>AMALTGCSEKININEDKISHKIDIPDSAWTIGIGEKFKNAGHPNVKYPMIDDSYVQGAPLGGFGAGTIGRTYNGGFSRWHLEIGKNKYTTVYANQFSVFQKVEGNKDGVAQVLYAGEPENGYLSSWKWDYPKESGMYYALYPNSWYTYTNKDLPVQLAVKQFSPIIPYNYKETSYPVAVFKWTAYNPTNKNVDVSIMFTWQNMIGFFGKQVNVNSGNFNKIIKDKSKDSEIVAAVMGNISNDNEEWNGEYSIGVKKVPGVDISYKAKFVTTGDGSDLWHEFSKNGILDNKDDETPTKQDGIGSAIAVNFKLQPGQTIEVPFALSWDLPIMKFGGGDKWYKMYTKYFGKNGKNSFAILKEALNNYQKWEKMIDDWQKPILSNKSKPDWYKTALFNELYYLADGGTAWENGKVGEKDKRTNNMFGLLECFDYNYYETLDVRFYGSFPLVMLWPDIEKQVMRQFADTINVQDSSEFKVGSNGAMAVKKVQGMIPHDLGSSYALPWIKINAYDWQNPNIWKDLNSKYVLLVYRDYVLTGKTDKEFLKYTWKSVKTALDKLKEMDKDNDGIPDNEGIPDQTYDTWSMKGTSAYCGSLWLAALKAAQEIGKVLKDNEAYIKYNEWYKIAQQNFEKELWNGEYYNFDTESDHKDSIMADQLAGQWYADILRLGDILPKDHVQKALKKIYEFNVMKFENGKMGAVNGMRPDGIVDESDIQAQEVWTGVTYALASFMKYRGMTEEAYNTAYGVYKMTYDKSGKGYWFRTPEAWTKDGNYRASMYMRPLSIWSMEVNYNEVLEHHHHHH[2x]

GBA2, the non-lysosomal β-glucosylceramidase, is an enzyme involved in glucosylceramide metabolism. GBA2, like TxGH116 (the bacterial homologue of GBA2), induces hydrolysis through the conventional Koshland two-step double-displacement conformational pathway typical of retaining β-glucosidases, progressing from 1S3 to 4H3 to ultimately adopt the 4C1 in the covalent complex. Very recent publication by Shimokawa and coworkers41 reports that a GH116 exo-β-d-arabino-furanosidase from Microbacterium arabinogalactanolyticum termed ExoMA2 shows similarities in structure to that of the GH116 β-glucosidase from Thermoanaerobacterium xylanolyticum (TxGH116). Both enzymes have a two-domain structure consisting of N-terminal β-sandwich and C-terminal (α/α) 6-barrel domains, the latter being the catalytic domain.

To firmly establish the mode of action of β-d-Araf cyclitol aziridines as mechanism-based GBA2 inhibitors, the 3-D structure of the GH116 bacterial GBA2 homolog, TxGH116 from Thermoanaerobacterium xylanolyticum in complex with β-d-Araf compound 2 was solved at 1.9 Å resolution. The −1 subsite of TxGH116 is well conserved relative to human GBA2. Electron density shows unambiguous covalent reaction of 2 with the catalytic nucleophile of TxGH116. Reacted compound 2 is anchored by several hydrogen bonds. The OH group on C2 interacts with NE2 His507 and OD2 Asp452, and the OH on C3 with OD2 Asp452, NH2 Arg792 and OG1 and the alcohol of Thr591. The OH on C5 is hydrogen-bonded to OE2 Glu777 and to NH1 and NH2 Arg786. In addition, the amine from the ring-opened aziridine group forms a hydrogen bond to OD2 Asp593 and to a water molecule (which also interacts with OD1 Asp593). There is insufficient electron density to allow modelling of the end of the octyl chain and the azido group, which extend into a more open region at the edge of the protein where they are less constrained. However, both the hydroxyl groups on C2 and C3 of the cyclophellitol-configured aziridine form hydrogen bonds to His507, whereas for 2, only a single hydrogen bond is possible with the side chain. In contrast to cyclophellitol aziridines, which mimic the 4H3 transition state, β-d-Araf aziridine adopts an 3E conformation34 which resembles the 1S3 initial Michaelis complex conformation.> UGGCUUAGAAGC;> GGCCGUAACUAUAACGGUC;> GCCCGUCACACCAUGGGAGUAUGACUGGG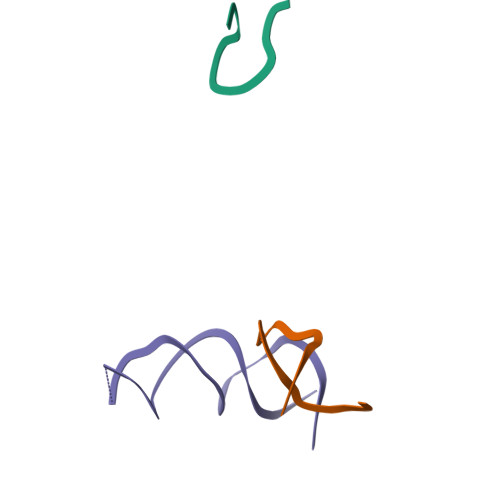GUGAAGUCGUAAC> GHMRSMVSKGEELIKENMRMKVVMEGSVNGHQFKCTGEGEGNPYMGTQTMRIKVIEGGPLPFAFDILATSFLYGSRTFIKYPKGIPDFFKQSFPEGFTWERVTRYEDGGV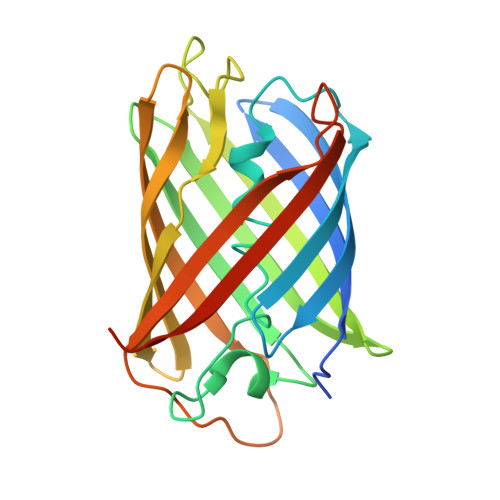VTVMQDTSLEDGCLVYHVQVRGVDFPSNGPVMQKKTKGWEPFTEMMYPADGGLRGYTHMALKVDGGGHLSCSFVTTYRSKKTVGNIKMPGIHAVDHRLERLEESDNEMFVVLREHSVAKFAGRGGMDELYK> TRRETQ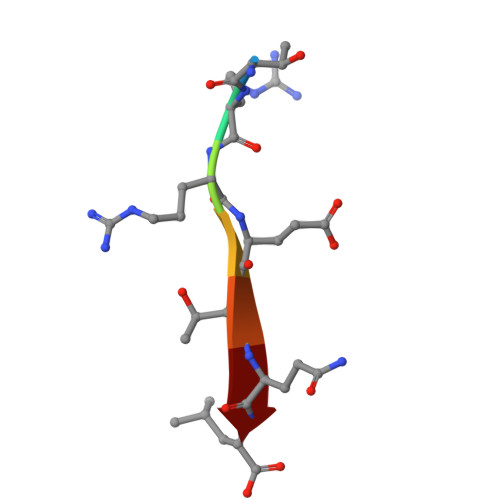L>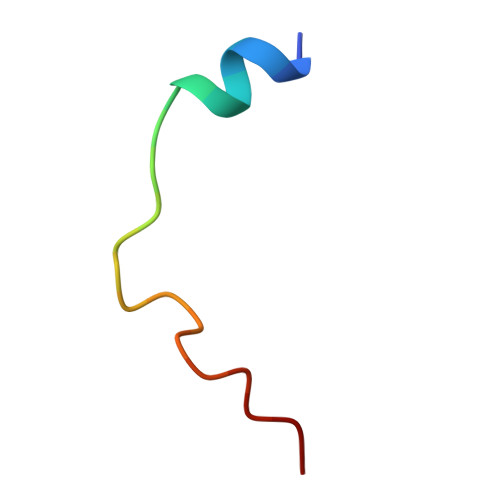 SWDSWFDGEGASTDFMSTREQP>MEQRASLDSEESESPPQENSCLDPPDRDPNCKPPPVKPHIFTTRSRTRLFGKGDSEEASPLDCPYEEGGLASCPIITVSSVLTIQRPGDGPASVRPSSQDSVSAGEKPPRLYDRRSIFDAVAQSNCQELESLLPFLQRSKKRLTDSEFKDPETGKTCLLKAMLNLHNGQNDTIALLLDVARKTDSLKQFVNASYTDSYYKGQTALHIAIERRNMTLVTLLVENGADVQAAANGDFFKKTKGRPGFYFGELPLSLAACTNQLAIVKFLLQNSWQPADISARDSVGNTVLHALVEVADNTVDNTKFVTSMYNEILILGAKLHPTLKLEEITNRKGLTPLALAASSGKIGVLAYILQREIHEPECRHLSRKFTEWAYGPVHSSLYDLSCIDTCEKNSVLEVIAYSSSETPNRHDMLLVEPLNRLLQDKWDRFVKRIFYFNFFVYCLYMIIFTAAAYYRPVEGLPPYKLKNTVGDYFRVTGEILSVSGGVYFFFRGIQYFLQRRPSLKSLFVDSYSEILFFVQSLFMLVSVVLYFSQRKEYVASMVFSLAMGWTNMLYYTRGFQQMGIYAVMIEKMILRDLCRFMFVYLVFLFGFSTAVVTLIEDGKNNSLPMESTPHKCRGSACKPGNSYNSLYSTCLELFKFTIGMGDLEFTENYDFKAVFIILL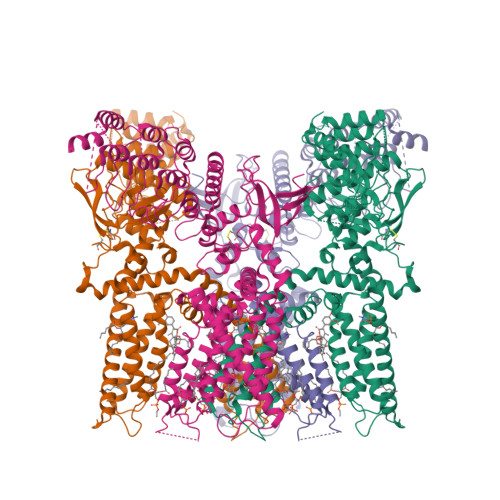LAYVILTYILLLNMLIALMGETVNKIAQESKNIWKLQRAITILDTEKSFLKCMRKAFRSGKLLQVGFTPDGKDDYRWCFRVDEVNWTTWNTNVGIINEDPGNCEGVKRTLSFSLRSGRVSGRNWKNFALVPLLRDASTRDRHATQQEEVQLKHYTGSLKPEDAEVFKDSMVPGEKENSLEVLFQGPDYKDDDDKAHHHHHHHHHH[4x]>MEKNSSPAETSGKQKVRSAEVGTDILKALAELSPATSLSRLAEHVGMPASKVHRYLQALIASGFAVQDASTNHYSLGREALRVGLAALDSMDVLKSAAAPLAELRDVLNETCFLAVWGNRGATVVQVEQAVRAVTVVTQVGSVLPLLGSSTGLVFAAFLPEREVAELREEELAGRADHPLADPAAYAVLLEGIRARGLHAIHGLLMPGVEALSAPVFDARGRVAAVLTVVGPASIFQAEEQGPAAERLLATTRAISWRMGYDGTQGG[2x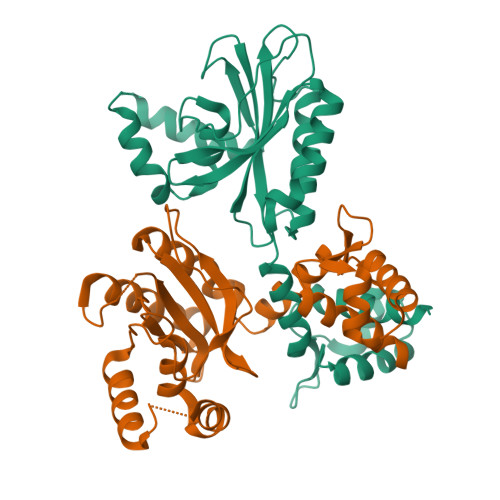]> GPLGSPEFMAQGTLIRVTPEQPTHAVCVLGTLTQLDICSSAPEDCTSFSINASPGVVVDIAHGPPAKKKSTGSSTWPLDPGVEVTLTMKVASGSTGDQKVQISYYGPKTPPVKALLYLTGVEISLCADITRTGKVKPTRAVKDQRTWTWGPCGQGAILLVNCDRDNLESSAMDCEDDEVLDSEDLQDMSLMTLSTKTPKDFFTNHTLVLHVARSEMDKVRVFQATRGKLSSKCSVVLGPKWPSHYLMVPGGKHNMDFYVEALAFPDTDFPGLITLTISLLDTSNLELPEAVVFQDSVVFRVAPWIMTPNTQPPQEVYACSIFENEDFLKSVTTLAMKAKCKLTICPEEENMDDQWMQDEMEIGYIQAPHKTLPVVFDSPRNRGLKEFPIKRVMGPDFGYVTRGPQTGGISGLDSFGNLEVSPPVTVRGKEYPLGRILFGDSCYPSNDSRQMHQALQDFLSAQQVQAPVKLYSDWLSVGHVDEFLSFVPAPDRKGFRLLLASPRSCYKLFQEQQNEGHGEALLFEGIKKKKQQKIKNILSNKTLREHNSFVERCIDWNRELLKRELGLAESDIIDIPQLFKLKEFSKAEAFFPNMVNMLVLGKHLGIPKPFGPVINGRCCLEEKVCSLLEPLGLQC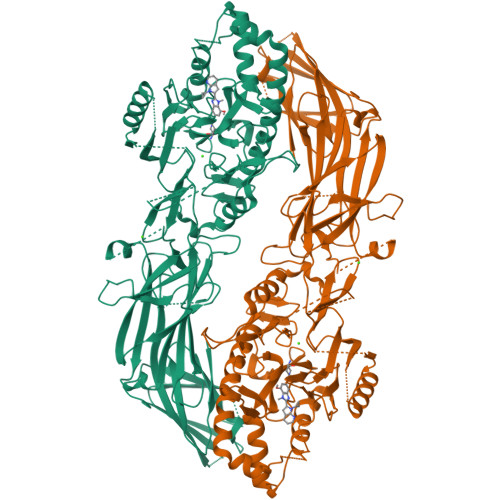TFINDFFTYHIRHGEVHAGTNVRRKPFSFKWWNMVP>[2x]VVGGTEAQRNSWPSQISLQYRSGSSWAHTCGGTLIRQNWVMTAAHCVDRELTFRVVVGEHNLNQNDGTEQYVGVQKIVVHPYWNTDDVAAGY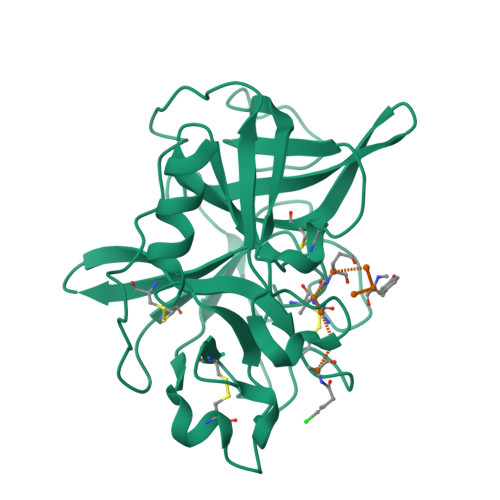DIALLRLAQSVTLNSYVQLGVLPRAGTILANNSPCYITGWGLTRTNGQLAQTLQQAYLPTVDYAICSSSSYWGSTVKNSMVCAGGDGVRSGCQGDSGGPLHCLVNGQYAVHGVTSFVSRLGCNVTRKPTVFTRVSAYISWINNVIASN>[3x]MAEYIKYRVPAKGVSATKGVAELIEKAEEEGIKTAWHRLLEQQPQCAFGQLGVCCRNCAMGPCRIDPFGSGPTKGVCGAGADTIVARNLLRMIAAGAAAHSDHARDVVEVFKGVAEGRFQYYKLTDVEKLKSLAETLGISTEGKDEHEIARELAEVLEWEFGKPGDEPLRMLALAPKKRIKVWEKAGVLPRAIDREVCECMHRTHIGVDADPVSLLLHGIRTSLADGWSGSMMATYLSDILFGTPKPLKAEANLGVLKEDYVNIVVHGHNPILSTKIAEIAMSEEMQKFAKKYGAKGVNVVGMCCTGNEVLMRLGVPIAGSFLMQELAIITGAVEAIIVDYQCIMPAIVDVAQCYHTKVITTEPKGHIPGAVHIE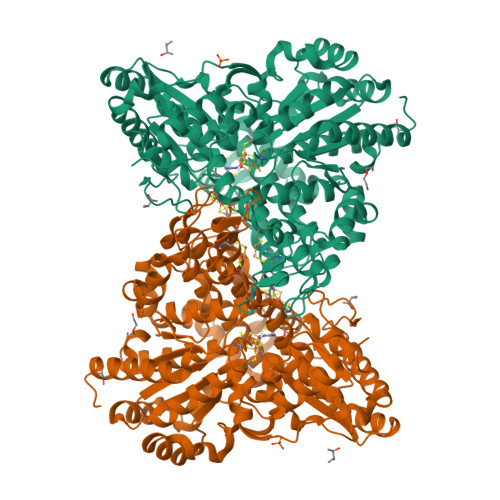FNAEKADEIAKEIVRIAIENYPNRPRDRVHIPKHKMEAIAGFSVEAIVEALGGTLEPLINALRDGTIKGIVGIVGCNNPKVKHNYSHVTLAKELIKRDVLVVGTGCWSIAAAMEGLMSPKAVDLAGPGLKKICEALNIPPCLHMGSCVDCSRILIALGALADALGVDISDLPAAGSAPEWMSEKAVSIGTYFVASGVFTHLGVVPPVMGSQKVAKILTEDVEDIIGGKFYVEPDPVKAAETIYNVILEKRKKLGWPL>[2x]GVEPQVGIVNGLAVYGPNSGSLLEIEVSVTAAQDKGSINITGIAEEESIGSQSKSIRRKSMAKGSVENVLTVLRTMGMKPSDYDIHINFPGGIPIDGPSAGIAMAAGIFSAIHKIPIDNTVAMTGEISLNGLVKPIGGVIPKIKAAKQSGAKKVIIPYENQQAILKQIDGIEIIAVKTFQEVLDEILVNPPTEQKPFHIEINKESV

ATP-dependent Lon proteases are key participants in the quality control system that supports the homeostasis of the cellular proteome. All Lons are single-chain, multidomain proteins containing an ATPase and protease domains, with different additional elements present in each subfamily. Primary structures of more than 100 Lon proteases from various organisms became available by the year 2000. Their comparative analysis showed that Lon proteases are non-classical serine peptidases, with catalytic centers formed by serine–lysine dyads. We thus postulate that this enzyme is the founding member of a newly identified LonBA subfamily, so far found only in the gene sequences of firmicutes.

The crystal structure of the P domain of BsLonBA (residues 347–552) was determined at the resolution of 1.9 Å. Crystals belong to the hexagonal space group P63 with two molecules (designated A and B) in the asymmetric unit, arranged around the crystallographic 3-fold axis. This arrangement results in the creation of an expected planar hexamer. The insertion of 14 residues (392–405) in the P domain of BsLonBA creates a 12-stranded β-barrel in the core of the hexameric assembly formed by β-hairpin inserts of the neighboring subunits (a detailed description below). Six inserts arranged around the three-fold symmetry axis complete a 12-stranded antiparallel β-barrel, where each insert forms nine hydrogen bonds with the neighboring subunit. We have captured the P domain in an inhibited state, in the complex with bortezomib, a covalently bound inhibitor. Bortezomib is covalently bound to the Oγ of Ser445 via the boronate moiety. Within the active site, bortezomib creates β-sheet-like interactions with residues of β1 (A359, V360, Y361) on one side, and residues of the loop β6-α3 (I441, D442) on the other side. Oxygen atoms of the boronate moiety make additional hydrogen bonds with the side-chain amine of Lys488 and the main chain nitrogen of Ser445. Analysis of the vicinity of the active site identified a putative sodium cation coordinated by carbonyl oxygens of Ser445 and Leu358, Oγ atoms of Thr470 and Ser445, and a water molecule.> MAHHHHHHMDNLLRHLKIS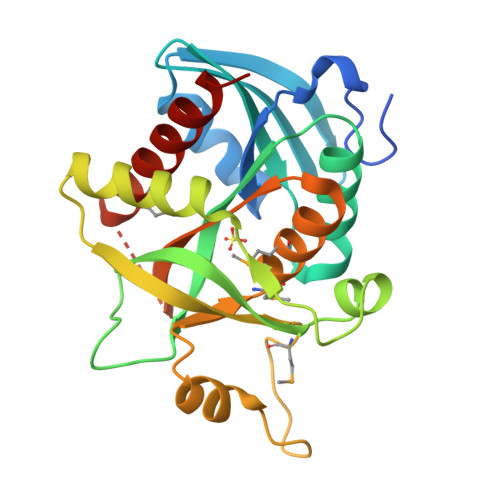KEQITPVVLVVGDPGRVDKIKVVCDSYVDLAYNREYKSVECHYKGQKFLCVSHGVGSAGCAVCFEELCQNGAKVIIRAGSCGSLQPDLIKRGDICICNAAVREDRVSHLLIHGDFPAVGDFDVYDTLNKCAQELNVPVFNGISVSSDMYYPNKIIPSRLEDYSKANAAVVEMELATLMVIGTLRKVKTGGILIVDGCPFKWDEGDFDNNLVPHQLENMIKIALGACAKLATKYA naphthalen-2-ylboronic acid | C10 H9 B O2 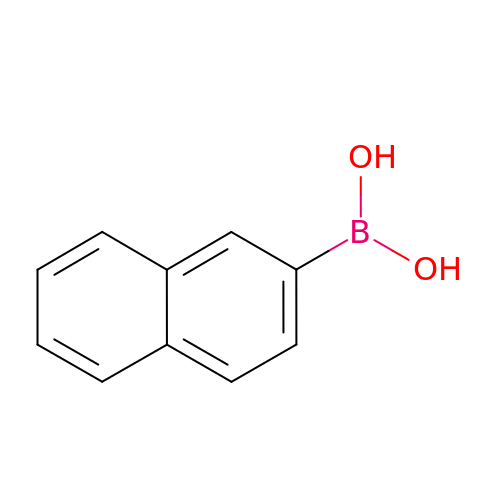| KPTRDYONBVUWPD-UHFFFAOYSA-N>GPSQNAIKRFMTLFSGREDVFSIQYEGGYRPIRRPLNFQDIKNHFSGKKTLGIYLLKKNDTVKFAAYDIDIKKHYLNREDKFVYEENSKKVAKRLSRELNLENITHYFEFTGNRGYHIWIFFDIPVSAYKIKYIMEKILDRI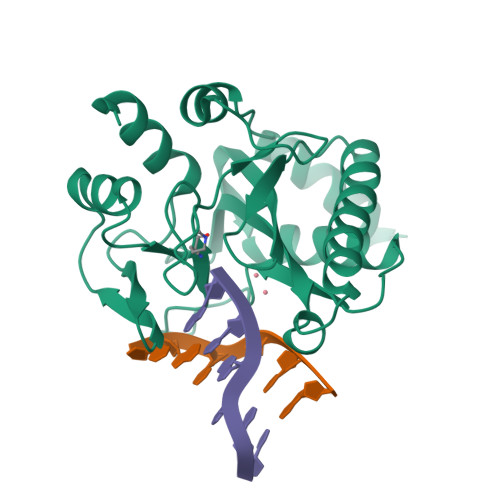ELEEGIDVEIFPKQTSLNGGLGNLIKVPLGVHKKTGKKCLFVDNDFNVIENQIEFLNNIKENKATEINKLFREIFNE[2x]>NQKYQALLANNVENTAKEALHQLAYTGREYNNIQDQIETISDLLGHSQSLYDYLREPSKANLTILENMWSSVARNQKLYKQIRFLDTSGTEKVRIKYDFKTSIAGPSLILRDKSAREYFKY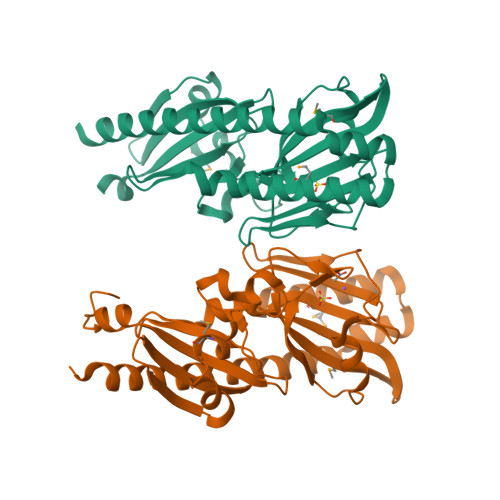AQSLDNEQISAWGIELERDKGELVYPLSPSLRILMPISVNDVRQGYLVLNVDIEYLSSLLNYSPVRDFHIELVKHKGFYIASPDESRLYGDIIPERSQFNFSNMYPDIWPRVVSEQAGYSYSGEHLIAFSSIKFVSNEPLHLIIDLSNEQLSKRATRDINDLIQES[2x]> DCNILQRLKVKMQWAKAYGFGTERAKFGN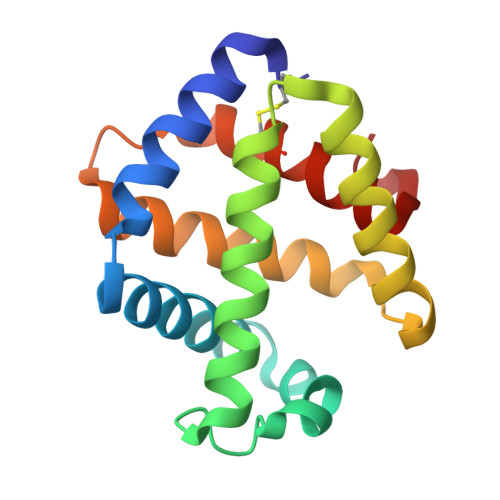SLWTSIFNYAPDARDLFKSVKSEDMRSPQFKAHIARVIGGLDRVISMFDNEDALNADLEHLKSQHDPRGLDALNFVVFGKALFATVGGQFGVCFDLPAWESCYKVIAMGITGNDMFS>XEVEALEKKVEALEAKVQKLEKKVEALEHGWDGR[2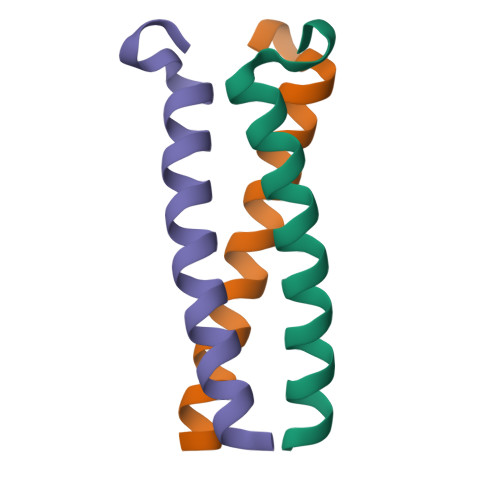x]2-(1H-BENZIMIDAZOL-2-YLSULFANYL)ETHANOL | C9 H10 N2 O S | 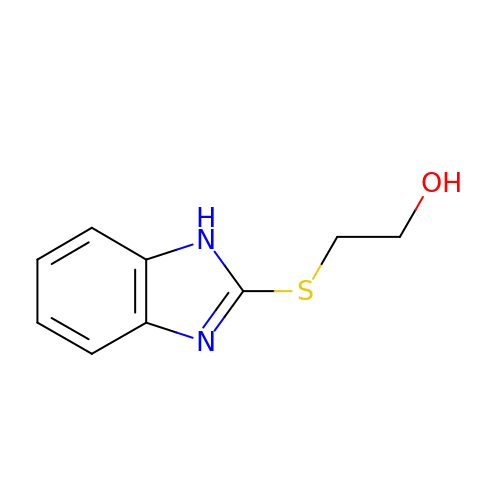HFDPECWVRWDXHN-UHFFFAOYSA-N> VEHISKGNNCLDAAKACNLDDTCKKYRSAYITPCTTSMSNEVCNRRKCHKALRQFFDKVPAKHSYGMLFCSCRDIACTERRRQTIVPVCSYEERERPNCLSLQDSC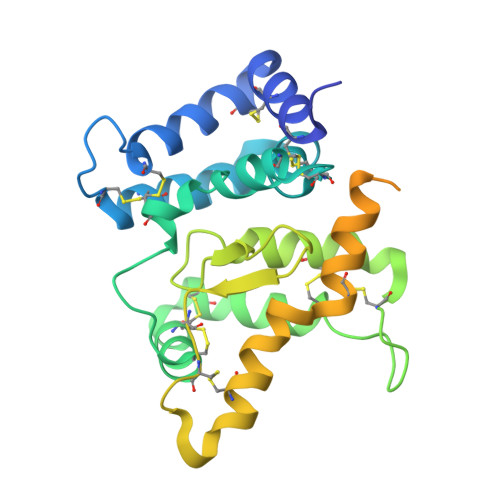KTNYICRSRLADFFTNCQPESRSVSNCLKENYADCLLAYSGLIGTVMTPNYVDSSSLSVAPWCDCSNSGNDLEDCLKFLNFFKDNTCLKNAIQAFGNGSDVTMWQPAPPVQTTTATTTTAFRVKNKPLGPAGSENEIPTHVLPPCANLQAQKLKSNVSGSTHLCLSDSDFGKDGL> GPLGSSACPSGATCGSYTVGGLGSRKQQVRNAGGSSLDLAVAMLETERMDTAYPYGDNKSGDAANFGIFKQNWLMLRSACAQFGGQGAGQYDNGAALNSSLGQDVSCLH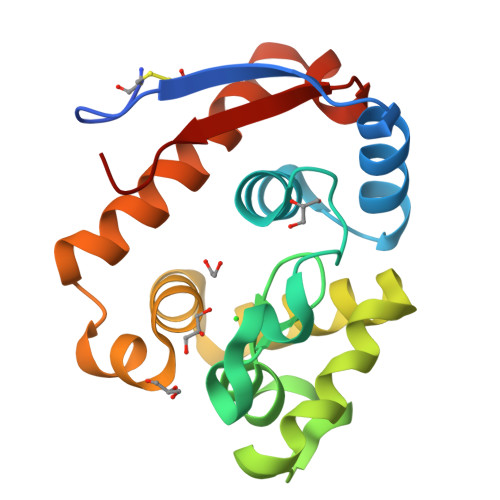QSQSHYGLDAWFAGHRNGASGLSSPNTADIAAYKAAVYWIKAQLDADSANLGNDTRFWVQVPAI> E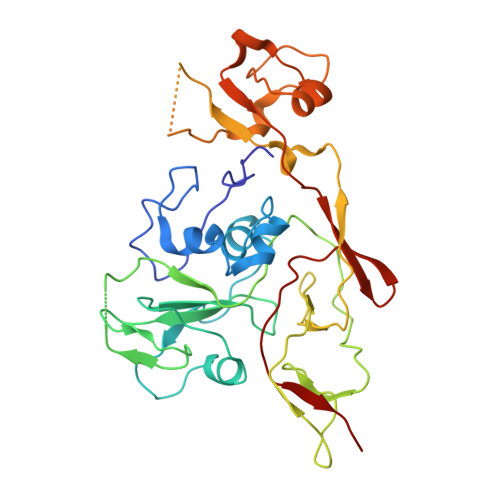DPHLRNRPGKGHNYIDGMTQEDATCKPVTYAGACSSFDVLLEKGKFPLFQSYAHHRTLLEAVHDTIIAKADPPSCDLQSAHGNPCMKEKLVMKTHCPNDYQSAHYLNNDGKMASVKCPPKYELTEDCNFCRQMTGASLKKGSYPLQDLFCQSSEDDGSKLKTKMKGVCEVGVQALKKCDGQLSTAHEVVPFAVFKNSKKVYLDKLDLKTEENLLPDSFVCFEHKGQYKGKLDSGQTKRELKSFDISQCPKIGGHGSKKCTGDAAFCSAYECTAQYANAYCSHANGSGIVQIQVSGVWKKPLCVGYERVVVKRELS>VSDALDEGLVQRIDARGTIEWSETCYRYTGAHRDALSGEGARRFGGRWNPPLLFPAIYLADSAQACMVEVERAAQAASTTAEKMLEAAYRLHTIDVTDLAVLDLTTPQAREAVGLENDDIYGDDWSGCQAVGHAAWFLHMQGVLVPA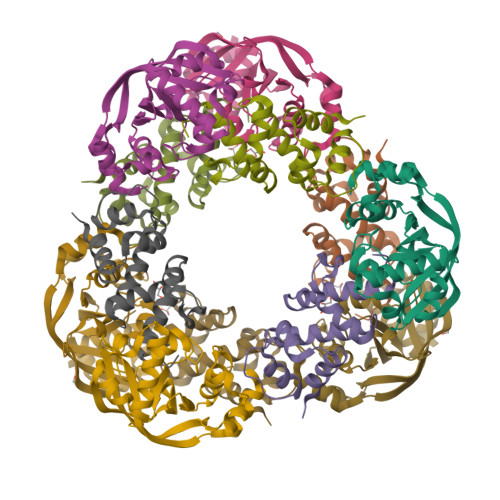AGGVGLVVTAYEQRTRPGQLQLRQSVDLTPALYQELRAT[2x];>[2x]GAMGVNVLASTVSGAIERLGLTYEEVGDIVDASPRSVARWTAGQVVPQRLNKQRLIELAYVADALAEVLPRDQANVWMFSPNRLLEHRKPADLVRDGEYQRVLALIDAMAEGVFV> KIKDPKILGIDPNVTQYTGYLDVEDEDKHFFFWTFESRNDPAKDPVILWLNGGPGCSSLTGLFFELGPSSIGPDLKPIGNPYSWNSNATVIFLDQPVNVGFSYSGSSGVSNTVAAGKDVYNFLELFFDQFPEYVNKGQDFHIAGESYAGHYIPVFASEILSHKDRNFNLTSVLIGNGLTDPLTQYNYYEPMACGEGGEPSVLPSEECSAMEDSLERCLGLIESCYDSQSVWSCVPATIYCNNAQLAPYQRTGRNVYDIRKDCEGGNLCYPTLQDIDDYLNQDYVKEAVGAEVDHYESCNFDINRNFLFAGDWMKPYHTAVTDLLNQDLPILVYAGDKDFICNWLGNKAWTDVLPWKYDEEFASQKVRNWTASITDEVAGEVKSYKHFTYLRVFNGGHMVPFDVPENALSMVNEWIHGGFSL;> XMNQAIDFAQASIDSYKKHGILEDVIHDTSFQPSGILAVEYSSSAPVAMGNTLPTEKARSKPQFQFTFNKQMQKSVPQANAYVPQDDDLFTLVMTDPDAPSKTDHKWSEFCHLVECDLKLLNEATHETSGATEFFASEFNTKGSNTLIEYMGPAPPKGSGPHRYVFLLYK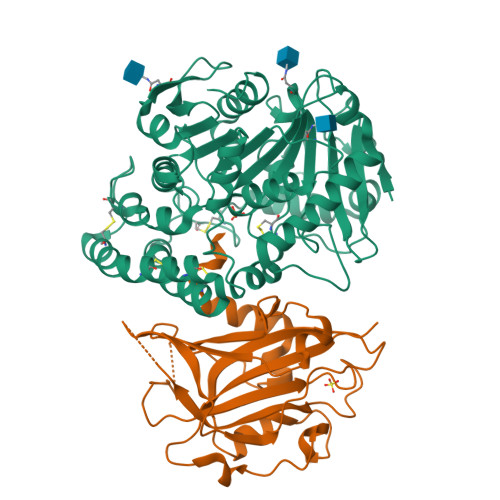QPKGVDSSKFSKIKDRPNWGYGTPATGVGKWAKENNLQLVASNFFYAETK> WSKEGHVMTCRIAQGLLNDEAAH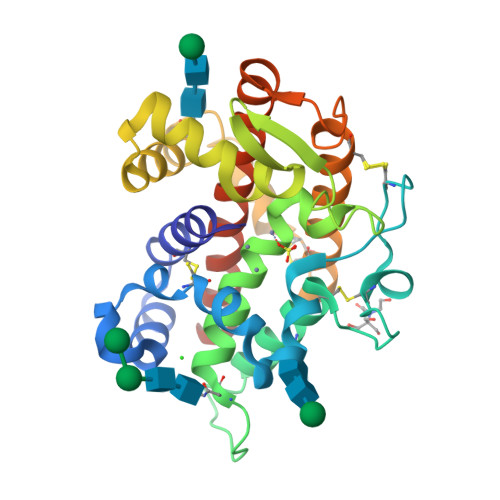AVKMLLPEYVNGDLSALCVWPDQVRHWYKYKWTSPLHFIDTPDKACNFDYERDCHDQHGVKDMCVAGAIQNFTTQLSHYREGTSDRRYNMTEALLFLSHFMGDIHQPMHVGFTSDAGGNSIDLRWFRHKSNLHHVWDREIILTAAKDYYAKDINLLEEDIEGNFTDGIWSDDLASWRECGNVFSCVNKFATESINIACKWGYKGVEAGETLSDDYFNSRLPIVMKRVAQGGIRLAMLLNNVFGASQQEDSVVAT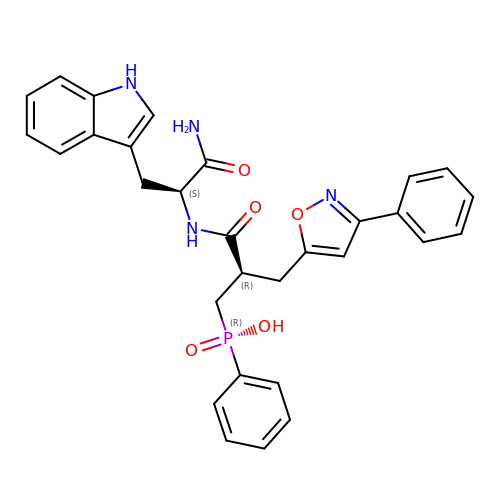NALPHA-{(2S)-3-[(S)-HYDROXY(PHENYL)PHOSPHORYL]-2-[(3-PHENYLISOXAZOL-5-YL)METHYL]PROPANOYL}-L-TRYPTOPHANAMIDE | C30 H29 N4 O5 P | NVKXUGMYWINPEL-DFHRPNOPSA-N> SGDGEGNVSDSVTLQDVLANDALVEFATDKNGCRFLQEHYPTENDNDVHQKLFRKLVEDRAIFLSLCSNMFGNFFVQRVLECSNTEEQEILTEHLATDLYNLCLDKSACRVIQLAIQKLDVHLATRLSLELRDTHLVRLSIDQNGNHVIQKIVKTLPVSSWTFLVDFFADDDNLIHVCQDKYGCRVIQSTVETLSTDQYAQCYQHRVILLRSLMAGVTRNCTQLASNEFANYVVQHVIKCGDALAVYRDIIIEQCLLQNLLSMSQE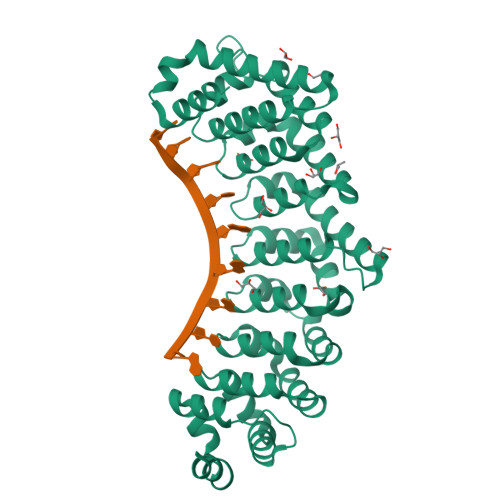KYASHVVEVAFECAPYRLVAEMMNEIFEGYIPHPDTNRDALDILLFHQYGNYVVQQMIQTCVLGQNARDQKQSEMYGMWLEKIHGRVMRNAHRLERFSSGKKIIEALQSMSLY> MKLQVLQVLDRLKMKLQEKGDTSQNEKLSMFYETLKSPLFNQILTLQQSIKQLK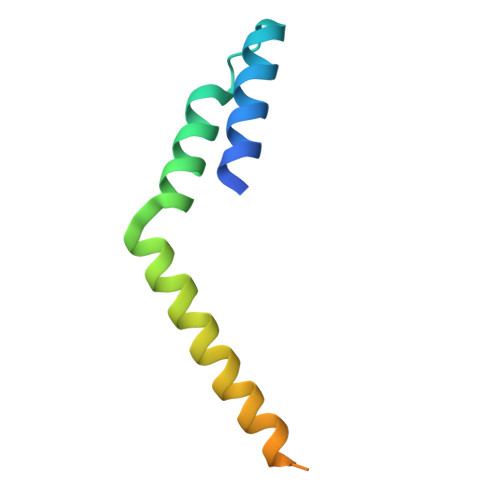GQLNHILESGKETAAAKFERQHMDSSTSA[(2~{R})-1-hexadecanoyloxy-3-[oxidanyl-[2-(trimethyl-$l^{4}-azanyl)ethoxy]phosphoryl]oxy-propan-2-yl] 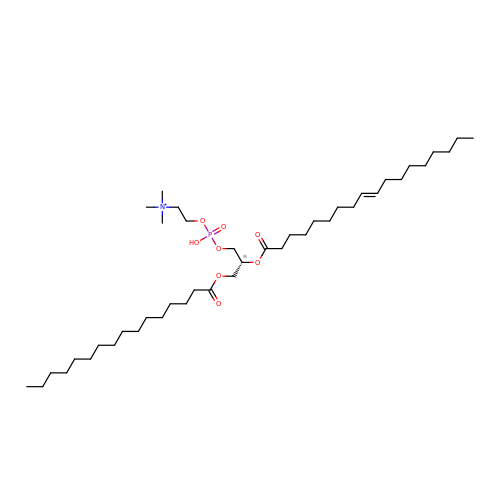octadec-9-enoate | C42 H83 N O8 P | BOJPVJHVFVFGBS-RRHRGVEJSA-N> GPYASLTEIEHLVQSVCKSYRETCQLRLEDLLRQRSNIFSREEVTGYQRKSMWEMWERCAHHLTEAIQYVVEFAKRLSGFMELCQNDQIVLLKAGAMEVVLVRMCRAYNADNRTVFFEGKYGGME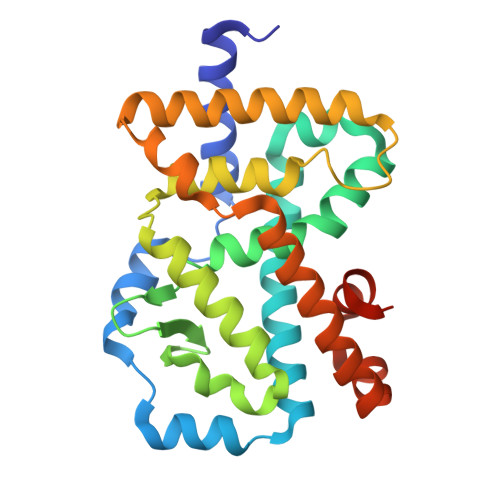LFRALGCSELISSIFDFSHSLSALHFSEDEIALYTALVLINAHRPGLQEKRKVEQLQYNLELAFHHHLSKTHRQSILAKLPPKGKLRSLCSQHVERLQIFQHLHPIVVQAAFPPLYKELFSTETESPVGLSK> NTYQFQNMIQCTVPKRSWRDFADYGCYCGRGGSGTPIDDLDSCCQVHDNCYNSAREQGG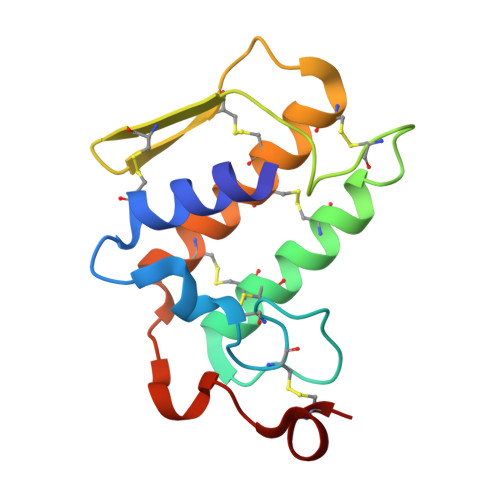CRPKQKTYTYQCKAGGLSCSGANNSCAATTCDCDRLAAICFAGAPYNDNNYNIDLKARCQ>[2x]MQKTLEVWIMPNSPQPAEDFKALVAPFEKAHGVEVKVTVLDWGVAWTKITTAATSGVGPDLTQLGTTWVGAISAMGVLEPVDDVLEALGGEKAYLPAVWRTTRLEGARQATAVPWFSELRAFYYRTDALKAAGVNPAEMFASWQGFEAGLARLKASSFRDPETKA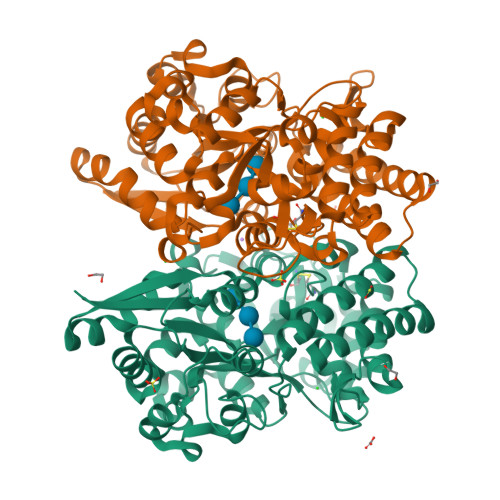PLAPLCTPGKNSWDVLHNAAPWIWGAGGEIVRQAGGRWQSALNSPESLEGLYFFLSLAQKGYVPAESLEKNTAQIEADFQAGKCAVFASGPWMIQRAQVPEAKGGFAERTAAKNLGVAPYPAGPKGRYTFFGGSNLALFNFSKNKPLAKELLKYLGGPEAQVRYAQMTGMLPALRSAWSDPSFQQNPLLRTFIQAAQFGRTYPSLAGWGGVENLAVQHLGMAWDLVAQGRLTREALKDLMDKASAAINQALRHHHHHH>EKVDNPFEGAKLYVNPVWSAKAAAEPGGSAVANESTAVWLDRIGAIEGNDSPTTGSMGLRDHLEEAVRQSGGDPLTIQVVIYNLPGRDC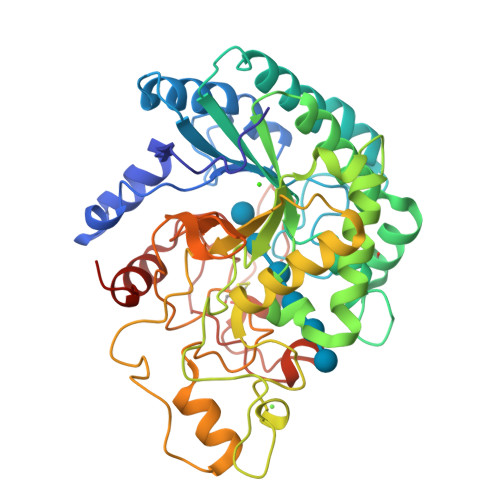AALASNGELGPDELDRYKSEYIDPIADIMWDFADYENLRIVAIIEIDSLPNLVTNVGGNGGTELCAYMKQNGGYVNGVGYALRKLGEIPNVYNYIDAAHHGWIGWDSNFGPSVDIFYEAANASGSTVDYVHGFISNTANYSATVEPYLDVNGTVNGQLIRQSKWVDWNQYVDELSFVQDLRQALIAKGFRSDIGMLIDTSRNGWGGPNRPTGPSSSTDLNTYVDESRIDRRIHPGNWCNQAGAGLGERPTVNPAPGVDAYVWVKPPGESDGASEEIPNDEGKGFDRMCDPTYQGNARNGNNPSGALPNAPISGHWFSAQFRELLANAYPPL[2x]>GSHMAQQNILSVHILNQQTGKPAADVTVTLEKKADNGWLQLNTAKTDKDGRIKALWPEQTATTGDYRVVFKTGDYF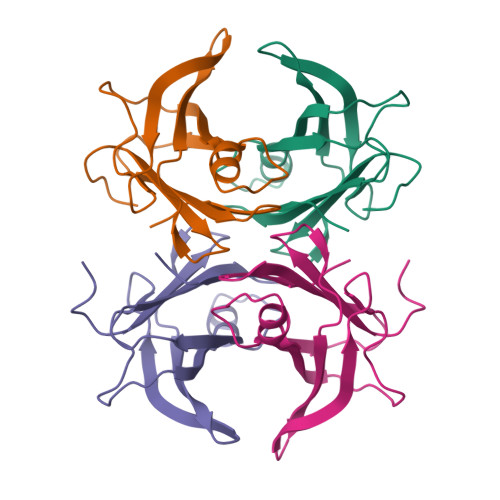KKQNLESFFPEIPVEFHINKVNEHYHVPLLLSQYGYSTYRGS[4x]THALASSOSPIRAMIDE C | 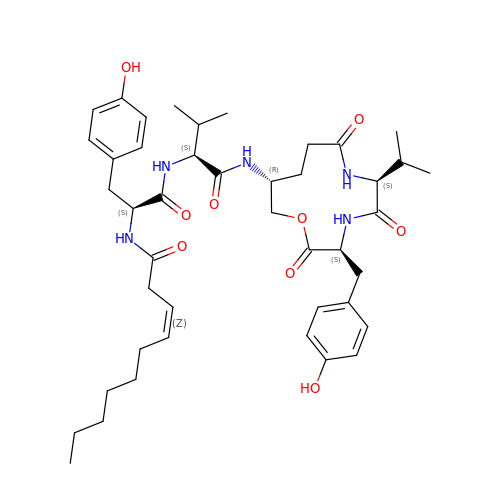C43 H61 N5 O9 | VEICWPPPDFDHMQ-GMWCJVCTSA-N N-{[4-({[(6R)-2-amino-5-formyl-4-oxo-1,4,5,6,7,8-hexahydropteridin-6-yl]methyl}amino)phenyl]carbonyl}-L-glutamic acid 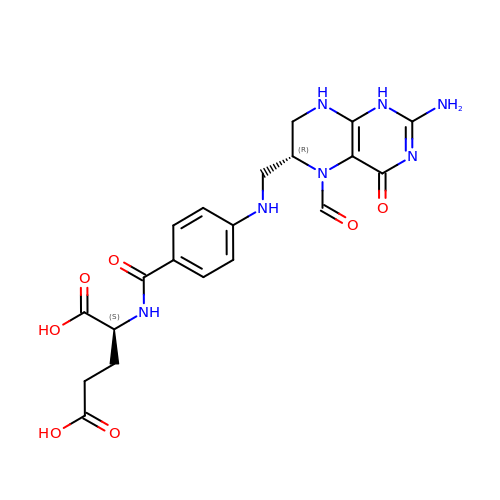| C20 H23 N7 O7 | VVIAGPKUTFNRDU-OLZOCXBDSA-N Upon contact with Langerhans cells, pathogens are captured by the C-type lectin langerin and internalized into a structurally unique vesicle known as a Birbeck granule. Langerin is a type II transmembrane protein that is composed of a cytoplasmic tail, coiled-coil neck region, and carbohydrate recognition domain (CRD) (Stambach and Taylor, 2003; Valladeau et al., 1999; Valladeau et al., 2000). Through the coiled-coil neck region, langerin forms a trimer, which is functionally important for oligosaccharide binding. The calcium-dependent carbohydrate-binding capacity of langerin CRD is essential for the formation of Birbeck granules because the removal of calcium ions causes them to unzip and disintegrate.

To purify these Birbeck granules, we expressed SNAP-tagged human langerin in 293T cells, biotinylated the tag by incubation with benzylguanine-biotin, and immunoprecipitated the Birbeck granules using streptavidin agarose. We conducted cryo-electron tomography of the isolated Birbeck granules and reconstructed the repeating units by averaging the subtomograms. The resolution was improved to 6.4 Å, which clearly visualized the alpha helices and enabled us to generate a model based on the previously reported crystal structure of the langerin trimer. We then performed a two-body refinement to visualize the spatial relationship between the two opposing langerin trimers. An in-depth analysis of the interaction region between the two CRDs revealed that the interaction is mediated by a loop at residues 258–263, which is highly flexible in the crystal structure. The interaction between the two CRDs appears to be maintained by docking the loops of two langerin molecules into each other’s lateral cleft, which constitutes the secondary carbohydrate-binding site (Figure 3A, pink circles; Chatwell et al., 2008). The interaction between the two CRDs is flexible because the first eigenvector of the multi-body analysis represents an approximately 30° tilting motion with the loop as the fulcrum. The docked loop 258–263 may provide additional interactions with the hydroxyl group of mannose via Glu261 and Asp263, thus increasing the affinity of the secondary binding site when two langerin trimers form a complex. To investigate the importance of loop 258–263 in the biogenesis of Birbeck granules, we mutated three residues in the loop: Met260Ala, Glu261Arg, and Asp263Lys, and generated three mutated langerin constructs, each carrying one (MRGD), two (MRGK), or three mutations (ARGK). In contrast, the internalization of the pseudovirus was significantly inhibited by the ARGK mutation. These results suggest that disruption of Birbeck granule formation by the mutation of loop 258–263 inhibited the internalization of HIV pseudovirus.

>[6x]MDKDCEMKRTTLDSPLGKLELSGCEQGLHEIKLLGKGTSAADAVEVPAPAAVLGGPEPLMQATAWLNAYFHQPEAIEEFPVPALHHPVFQQESFTRQVLWKLLKVVKFGEVISYQQLAALAGNPAATAAVKTALSGNPVPILIPCHRVVSSSGAVGGYEGGLAVKEWLLAHEGHRLGKPGLGPAGYPYDVPDYAYPYDVPDYAYPYDVPDYAGSSGLEVLFQGPTVEKEAPDAHFTVDKQNISLWPREPPPKSGPSLVPGKTPTVRAALICLTLVLVASVLLQAVLYPRFMGTISDVKTNVQLLKGRVDNISTLDSEIKKNSDGMEAAGVQIQMVNESLGYVRSQFLKLKTSVEKANAQIQILTRSWEEVSTLNAQIPELKSDLEKASALNTKIRALQGSLENMSKLLKRQNDILQVVSQGWKYFKGNFYYFSLIPKTWYSAEQFCVSRNSHLTSVTSESEQEFLYKTAGGLIYWIGLTKAGMEGDWSWVDDTPFNKVQSARFWIPGEPNNAGNNEHCGNIKAPSLQAWNDAPCDKTFLFICKRPYVPSEP Herein, we provide high‐resolution structures for an EAL enzyme Bd1971, from the predatory bacterium Bdellovibrio bacteriovorus, which is controlled by a second signaling nucleotide, cAMP. The Bd1971 domain architecture is predicted to consist of an N‐terminal cNMP sensory domain (cyclic nucleotide monophosphate, postulated to bind cAMP or cGMP), a middle linker region, and C‐terminal catalytic EAL barrel. We reveal that regulation of c‐di‐GMP hydrolysis arises from a domain‐swapping of the “regular” cNMP fold, which undergoes significant rearrangements upon binding of stimulus, communicating a series of conformational changes over 40 Å to license a productive state at the EAL dimer interface. C‐di‐GMP turnover was increased ~8‐fold in the presence of cAMP or cGMP, further supporting the proposal that cNMPs are activators of Bd1971.

To gain insight into the mode of allosteric regulation, we therefore designed a truncation mutant (residues 1–150, referred to hereafter as Bd1971ΔEAL, truncated at the point which the linker helix no longer contacts the cNMP sensor domain) that was amenable to study. The structure of the Bd1971ΔEAL construct was determined to 2.45 Å resolution, enabling us to trace residues 4–111 of the sensor‐hinge–C‐helix region of the protein. This truncated variant retains the CRP variant dimer interface observed in the full‐length protein and has two clearly empty cNMP sensor domains. The Bd1971ΔEAL structure reveals that the relationship between the cNMP body and hinge/C‐helix dimer interface has changed relative to that of the full‐length cAMP‐bound form, such that the apo/bound structures can be superimposed on one of these elements but not both. This conformational change upon losing ligand is best described by the realization that the C‐helix interface is essentially unchanged (between apo and bound states), and acts as a stator to allow the cNMP body to swing‐out relative to the central twofold axis. Alignment of the bound and apo‐forms using the C‐helix interface (residues 97–110 of both chains) reveals that the cNMP body rotates ~50° relative to the plane between the C‐helices. Residues 81‐86 spanning the connection between the cNMP body and hinge helix comprise the fulcrum for this motion (identified using DynDom; Girdlestone & Hayward, 2016, labeled “cNMP link” in Fig 6B and C), resulting in the largest translation between apo and bound structures occurring at the distal end of the fold (the β‐hairpin element of the cNMP body shifts 25 Å, as depicted by an arrow in Fig 6A). The concerted rotation and translation of the cNMP fold places the outer face of the β‐sandwich (strands 1, 3, 6, and 8) into an orientation that would sterically clash with the linker helix of the opposing chain in the cAMP‐bound full‐length structure.

>AAQSVDIHKDQIIFSEGDAGDCAYIIEKGRVLIYLTKDKEEIPLTILGEGEIFGEMALIDNQNRSASVRALEDVRLAIVTKQQVLERVSTADKVVQLLMRVLLKRLRR[2x]> MEVRKVIAAGEVIESPVDVVKELVENSLDAKATKVEVEIVKGGKRLIRVKDNGTGIHPEDVEKVVLQGATSKIETEKDLMNISTYGFRGEALYSISSVSKFKLRSRFFQEKEGKEIEVEAGNILGTRRVGMPVGTEVEVRDLFFNLPVRRKFLKKEDTERRKVLELIKEYALTNPEVEFTLFSEGRETLKLKKSSLKERVEEVFQTKTEELYAEREGITLRAFVSRNQRQGKYYVFINKRPIQNKNLKEFLRKVFGYKTLVVLYAELPPFMVDFNVHPKKKEV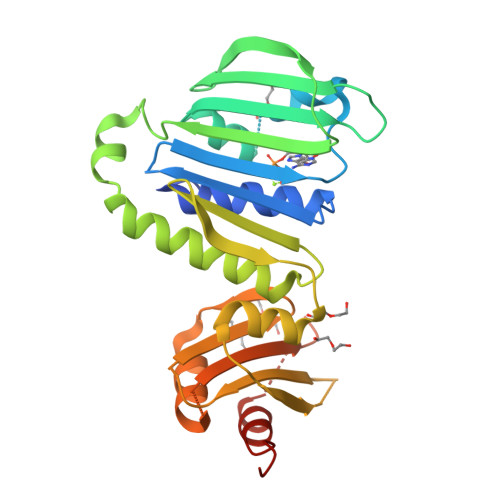NILKERKFLELVRELAGKEKPIVDI>MRSVASDREVRGPASTEEELSAVLTSIDSSAIASNIQHHADFTPLFSPEHSSPLKAYHATAKSVFDSLIMNWNATYDYYNKVNAKQAYYLSMEFLQGRALTNAIGNLELTGQYAEALKQLGHNLEDVASQEPDPALGNGGLGRLASCFLDSLATLNYPAWGYGLRYRYGLFKQIITKDGQEEVAENWLEMGNPWEIVRNDVSYPVKFYGKVVEGTDGRKHWIGGENIKAVAHDVPIPGYKTKTTNNLRLWSTTVPSQNFDLGAFNAGDHAKANEAHLNAEKICHVLYPGDESSEGKILRLKQQYTLCSASLQDIISRFESRAGDSLNWEDFPSKVAVQMNDTHPTLCIPELMRILMDIKGLSWNEAWSITERTVAYTNHTVLPEALEKWSLDIMQKLLPRHVEIIETIDEELMNNIVSKYGTADISLLKQKLKDMRILDNVDLPASVAKLFIKPKEKRGKLLVESLESIAEADEKTESQEVENILSETTEKKAESDSEEAPDAEKEDPEYELDPFAKYDPQFPRVVRMANLCVVGGHSVNGVAEIHSEIVKQDVFNSFYEMWPTKFQNKTNGVTPRRWIRFCNPELSTIISKWIGSDDWILNTDKLAGLKKFADDEDL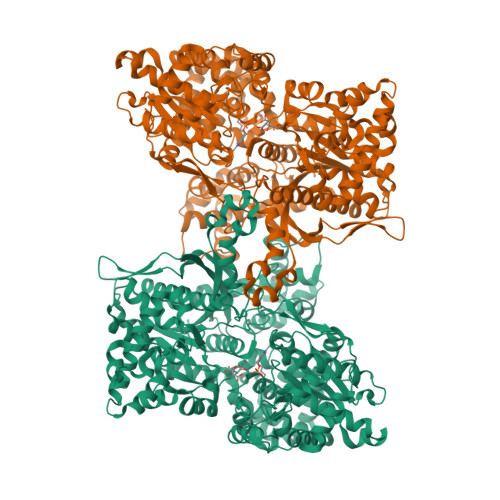QSEWRTAKRNNKMKVVSLIRDKTGYIVSPDAMFDVQVKRIHEYKRQLLNILGIVYRYKKMKEMSAKDRRKSFVPRVCIFGGKAFATYVQAKRIVKFITDVAATVNYDPDIGDLLKVVFVPDYNVSVAETLIPASELSQHISTAGMEASGTSNMKFAMNGCLLIGTLDGANVEIREEVGEENFFLFGAHAPEIAGLRQERAEGKFVPDLRFEEVKEYVRSGVFGTSNYDELMGSLEGNEGYGRADYFLVGKDFPSYIECQEKVDEAYRDQKLWTRMSILNTAGSPKFSSDRTIHEYAKDIWDISPVIMPTFPDIENLYFQG[2x]The oxidative degradation pathway of camphor requires two enantiocomplementary type II BMVOs, 2,5-diketocamphane 1,2-monooxygenase (2,5-DKMO; EC 1.14.13.162) and 3,6-diketocamphane 1,6-monooxygenase (3,6-DKMO; EC 1.14.13.–), which catalyse the NADH-dependent lactonization of diketocamphane stereoisomers (2,5- and 3,6-diketocamphane). Type II BVMOs utilize a FMN cofactor, which is reduced by a separate NADH dehydrogenase enzyme. The three-dimensional structures of the native enzyme and the FMN complex of the overexpressed form of the oxygenating component of the type II Baeyer–Villiger 3,6-diketocamphane monooxygenase have been determined to 1.9 Å resolution. The 3,6-DKMO monomer is made up from a single domain with an eight-stranded α/β-barrel (TIM-barrel) fold which has the nonprolyl cis-residue Ala77 forming a β-bulge in the middle of β-strand 3.

Initial structural characterization studies of 3,6-DKMO by our group were with the native enzyme purified from camphor-induced P. putida cell cultures. The native 3,6-DKMO crystallized in space group P212121, with unit-cell parameters a = 55.0, b = 93.4, c = 162.0 Å. The crystals that were grown in 50 mM PIPES pH 6.5, 50% ammonium sulfate contained two DKMO subunits in the asymmetric unit with a solvent content of 50%. The native 3,6-DKMO model also contains 798 water molecules, several glycerol molecules, four sulfate ions and two PIPES buffer molecules. The two subunits of the native structure were rebuilt independently. The root-mean-square deviation (r.m.s.d.) between Cα positions of the two subunits is 0.23 Å. In the course of the purification of the 3,6-DKMO enzyme the cofactor FMN is easily lost, especially if an ammonium sulfate precipitation step is used in the purification procedure, since the inorganic sulfate competes for the cofactor-binding site. The following residues were not modelled owing to disorder: A1, A128–133, A176–180, A377–378, B1, B127–135 and B176–179 in the native structure and A126–135, A176–179, A377–378, B125–135 and B176–179 in the FMN-complex structure.

>[2x]MAMETGLIFHPYMRPGRSARQTFDWGIKSAVQADSVGIDSMMISEHASQIWENIPNPELLIAAAALQTKNIKFAPMAHLLPHQHPAKLATMIGWLSQILEGRYFLGIGAGAYPQASYMHGIRNAGQSNTATGGEETKNLNDMVRESLFIMEKIWKREPFFHEGKYWDAGYPEELEGEEGDEQHKLADFSPWGGKAPEIAVTGFSYNSPSMRLAGERNFKPVSIFSGLDALKRHWEVYSEAAIEAGHTPDRSRHAVSHTVFCADTDKEAKRLVMEGPIGYCFERYLIPIWRRFGMMDGYAKDAGIDPVDADLEFLVDNVFLVGSPDTVTEKINALFEATGGWGTLQVEAHDYYDDPAPWFQSLELISKEVAPKILLPKR>KEENNFINLYTVKNPLKCKIVDKINLVRPNSPNEVYHLEINHNGLFKYLEGHTCGIIPYYNELDNNPNNQINKDHNIINTTNHTNHNNIALSHIKKQRCARLYSISSSNNMENLSVAIKIHKYEQTENAPNITNYGYCSGFIKNLKINDDIYLTGAHGYFNLPNDAIQKN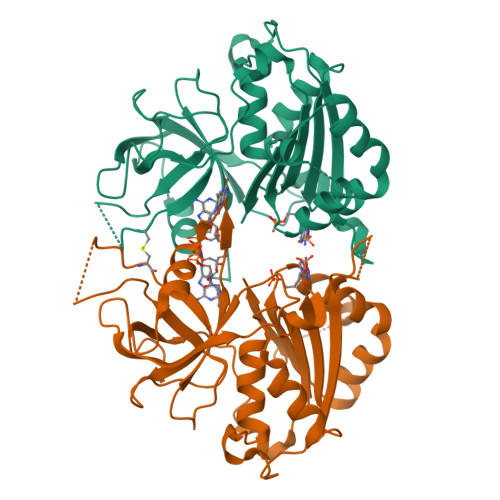TNFIFIATGTGISPYISFLKKLFAYDKNNLYNRNSNYTGYITIYYGVYNEDSILYLNELEYFQKMYPNNINIHYVFSYKQNSDATSFYVQDEIYKRKTEFLNLFNNYKCELYICGKKSIRYKVMDILKSHDQFDEKKKKRVHVEVY[6x]At the inner surface of fly photoreceptor rhabdomeric membranes, the master scaffold protein INAD (encoded by inaD for inactivation no after potential D and contains 5 PDZ domains arranged in tandem) forms stoichiometric multi-molecular complexes with phospholipase Cβ (NORPA), Ca2+-permeable transient receptor potential (TRP) channel and eye-specific protein kinase C (eye-PKC). In this study, we show that the PDZ45 tandem of INAD functions as a supramodule binding to the entire C-terminal coiled-coil domain and PDZ-binding motif of NORPA (CC-PBM) with an unexpectedly high affinity. Our biochemical and structural studies demonstrate that INADL PDZ89 forms a supramodule and binds to the entire C-terminal coiled-coil domain of PLCβ4 in a manner that is strikingly similar to that of the INAD–NORPA complex. The striking similarity between the PDZ scaffold and PLCβ interactions at the molecular level might point to an evolutionarily conserved molecular adaption in PLCβ signaling in the animal kingdom.

Like the coiled-coil structure of mammalian PLCβ3, NORPA CC folds into an elongated three helix bundle structure with an N-terminal short helix coupling to the middle region of the helix bundle. The packing surface of NORPA CC-PBM crystals involves an extensive surface composed of α1–α4. We reasoned that this packing surface might overlap with the INAD PDZ45 binding surface, and therefore prevented the same surface from being used for crystal packing in the PDZ45–NORPA CC-PBM complex. We noted that the solvent-exposed face of the α2 helix is lined with eight Lys residues, which are all evolutionarily conserved and required for the membrane binding of NORPA CC (and see below for more details). The evolutionarily conserved, positively charged residues in the α2 helix of the NORPA CC are aligned on a flat and exposed surface of the domain.

>EPPLVFEPVTLESLRQEKGFQEVGKKQIKELDTLREKHAKERTSVQKTQNAAIDKLIKGKSKDDIRNDANIKNSINDQTKQWTDMIARHRKEEWDMLRQHVQDSQDAMKALMLTVQAAQIKQLEDRHARDIKDLNAKQAKMSADTAKEVQNDTLKTKNEKDRRLREKRQNNVKRFMEEKKQIGVKQGRAMEKLKLAHSKQIEEFSTDVQKL[2x]~{N}-[6-methyl-5-[3-[2-[[(3~{S})-piperidin-3-yl]amino]pyrimidin-4-yl]pyridin-2-yl]oxy-naphthalen-1-yl]but-2-ynamide | C29 H28 N6 O2 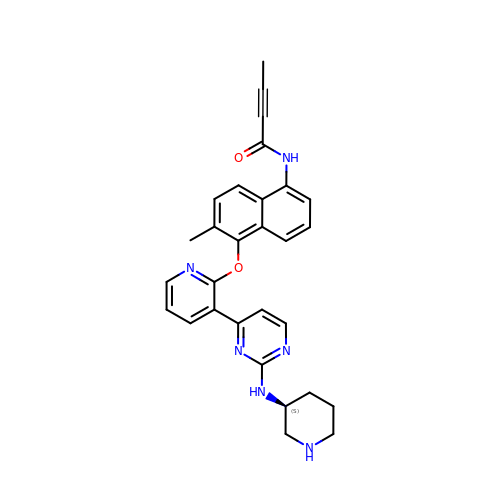| NYJNJBQWBJXYJJ-FQEVSTJZSA-N>GSDDELLYLPVRGRETYEMLLKIKESLELMQYLP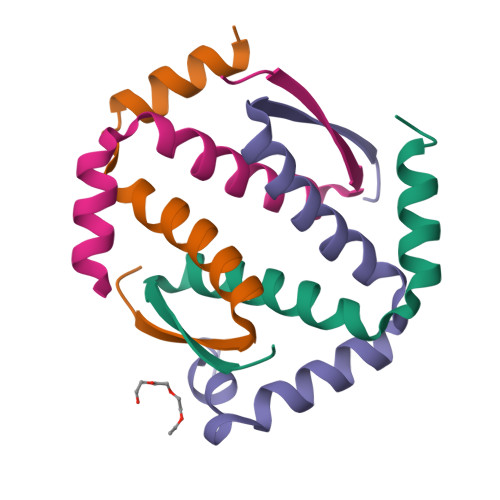QHTIETYRQQQQQQHQHLLQKQTSIQS[4x]>MKAAVVEQFKEPLKIKEVEKPTISYGEVLVRIKACGVCHTDLHAAHGDWPVKPKLPLIPGHEGVGIVEEVGPGVTHLKVGDRVGIPWLYSACGHCDYCLSGQETLCEHQKNAGYSVDGGYAEYCRAAADYVVKIPDNLSFEEAAPIFCAGVTTYKALKVTGAKPGEWVAIYGIGGFGHVAVQYAKAMGLNVVAVDIGDEKLELAKELGADLVVNPLKEDAAKFMKEKVGGVHAAVVTAVSKPAFQSAYNSIRRGGACVLVGLPP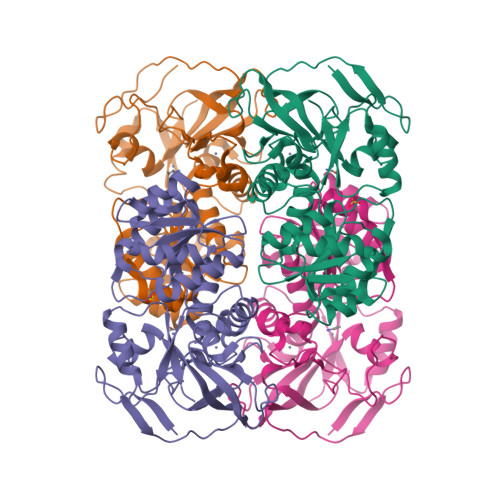EEMPIPIFDTVLNGIKIIGSIVGTRKDLQEALQFAAEGKVKTIIEVQPLEKINEVFDRMLKGQINGRVVLTLEDK[4x]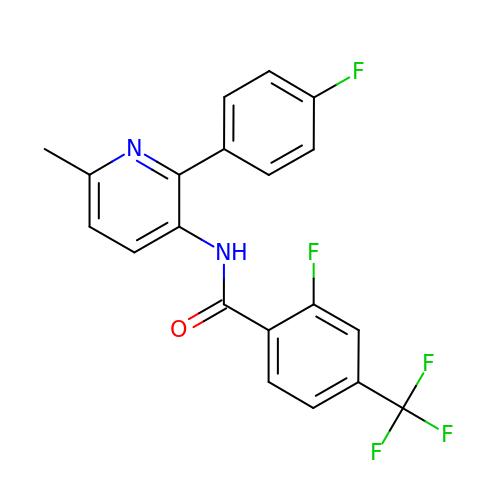2-fluoranyl-~{N}-[2-(4-fluorophenyl)-6-methyl-pyridin-3-yl]-4-(trifluoromethyl)benzamide | C20 H13 F5 N2 O | FBACRSKJFHDTDV-UHFFFAOYSA-N>MLFGIGLMPHGNPALSPEDKETEKLAGVLKDIGKAFSDADSYVLISPHNVRISDHLGVIMAQHLISWLGFEGVELPGEWETDRGLAEEVYNAWKGAEIPTVDLHFASRSGRYSRWPLTWGELIPLQFLEKKPLVLLTPARRLSRETLIKAGEVLGEVLEGSEKKIA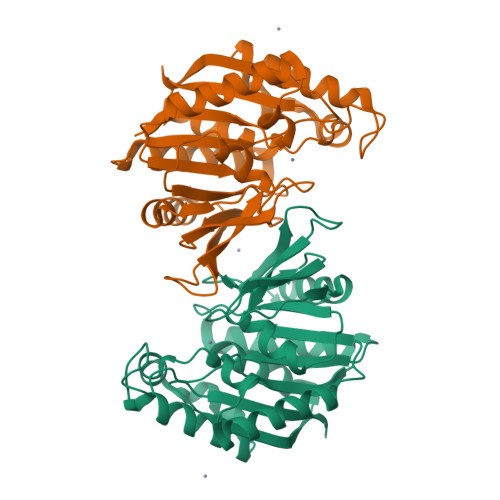LIVSADHGHAHDENGPYGYRKESEEYDRLIMELINESRLEELPEIPDELIEKALPDSYWQMLIMLGAMHRVPVKLVESAYACPTYFGMAGALWVRE[2x]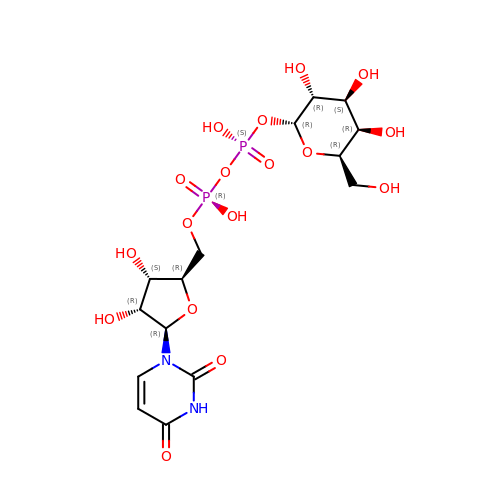GALACTOSE-URIDINE-5'-DIPHOSPHATE | C15 H24 N2 O17 P2 | HSCJRCZFDFQWRP-ABVWGUQPSA-N>GPHMKHPLMNVWTLWYLENDR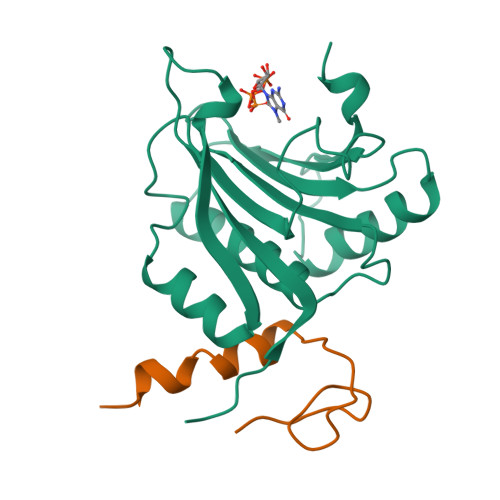SKSWEDMQNEITSFDTVEDFWSLYNHIKPPSEIKLGSDYSLFKKNIRPMWEDAANKQGGRWVITLNKSSKTDLDNLWLDVLLCLIGEAFDHSDQICGAVINIRGKSNKISIWTADGNNEEAALEIGHKLRDALRLGRNNSLQYQLHKDTMVKQGSNVKSIYTL[2x];> GHMLEPETTLNDKQDSTDLKVKVSAKISSIINYNEGQWSPNNPSGKKQYDREQLLQLREVKASRIQPEVKNVSILPQP>[2x]GSHMKIRQRFRFGRLELKRISGRGFKNDEEILIGNGTIQKIGIWD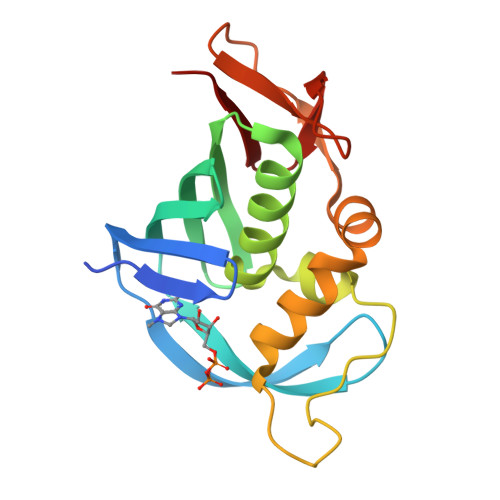GEEEFHVRCGECRGILKKSKMKLEKLLINSAKKEDMRDLIILCMVFSQDTRMFQGVRGEINFLNRAGQLLSPMYQLQRYFLNRSSDLFDQWGYEESPKASELHGINESMNASDYTLKGVVVTKN>[2x]SIISRSTFEEMLKHRNDAACPAKGFYTYDAFISAAKAFPAFG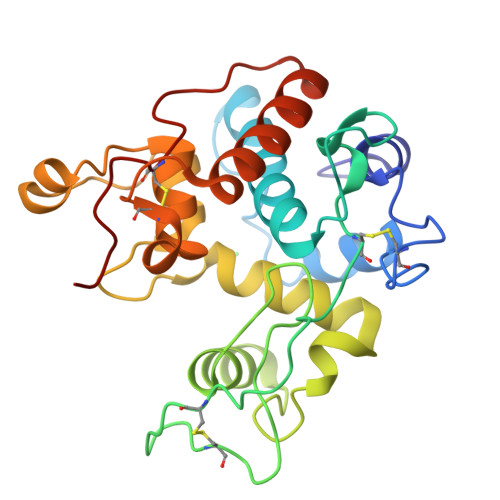TTGDVDTCKREIAAFFGQTSHATTGGWPTAPDGPYAWGYCYKEELNQASSYCSPSPAYPCAPGKKYYGRGPIQLSWNYNYGQCGQALGLDLLNNPDLVATDRVISFKAAIWFWMTPQFPKPSCHDVITGQWSPTGHDISAGRAPGYGVITNIINGGLECGRGWDARVEDRIGFYKRYCDMFAVGYGSNLDCYNQTPFGLG> DIFEAQKIEWHEGAHM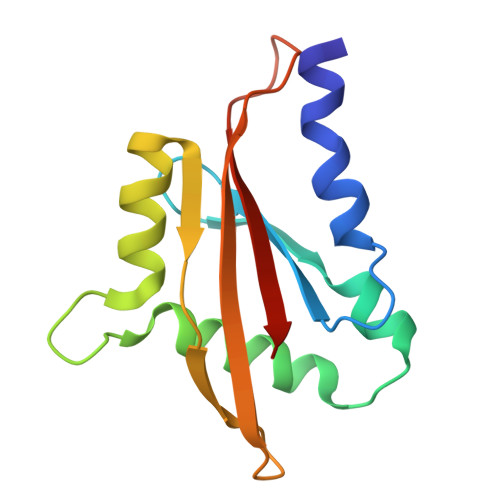TGVESFMTKQDTTGKIISIDTSSLRAAGRTGWEDLVRKCIYAFFQPQGREPSYARQLFQEVMTRGTASSPSYRFILNDGTMLSAHTKCKLCYPQSPDMQPFIMGIHIIDRE>EYNAPSEIKYIDVVNTYDLEEEASKVVPHGGFNYIAGASGDEWTKRANDRAWKHKLLYPRLAQDVEAPDTSTEILGHKIKAPFIMAPIAAHGLAHTTKEAGTARAVSEFGTIMSISAYSGATFEEISEGLNGGPRWFQIYMAKDDQQNRDILDEAKSDGATAIILTADSTVSGNRDRDVKNKFVYPFGMPIVQRYLRGTAEGMSLNNIYGASKQKISPRDIEEIAGHSGLPVFVKGIQHPEDADMAIKRGASGIWVSNHGARQLYEAPGSFDTLPAIAERVNKRVPIVFDSGVRRGEHVAKALASG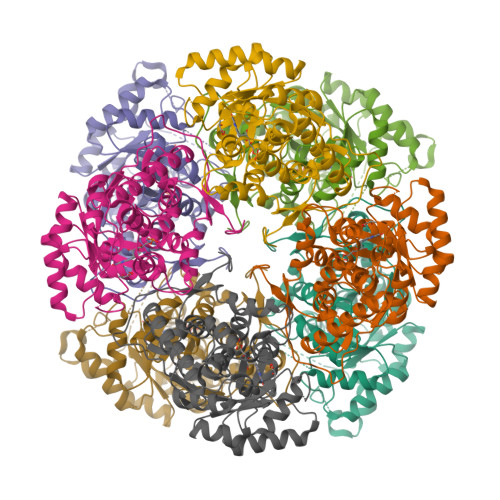ADVVALGRPVLFGLALGGWQGAYSVLDYFQKDLTRVMQLTGSQNVEDLKGLDLFDNPYGYEY[2x]>MDYPDPDTIRILITTDNHVGYNENDPITGDDSWKTFHEVMMLAKNNNVDMVVQSGDLFHVNKPSKKSLYQVLKTLRLCCMGDKPCELELLSDPSQVFHYDEFTNVNYEDPNFNISIPVFGISGNHDDASGDSLLCPMDILHATGLINHFGKVIESDKIKVVPLLFQKGSTKLALYGLAAVRDERLFRTFKDGGVTFEVPTMREGEWFNLMCVHQNHTGHTNTAFLPEQFLPDFLDMVIWGHEHECIPNLVHNPIKNFDVLQPGSSVATSLCEAEAQPKYVFILDIKYGEAPKMTPIPLETIRTFKMKSISLQDVPHLRPHDKDATSKYLIEQVEEMIRDANEETKQKLADDGEGDMVAELPKPLIRLRVDYSAPSNTQSPIDYQVENPRRFSNRFVGRVANGNNVVQFYKKRSPVTRSKKSGINGTSISDRDVEKLFSESGGELEVQTLVNDLLNKMQLSLLPEVGLNEAVKKFVDKDEKTALKEFISHEISNEVGILSTNEEFLRTDDAEEMKALIKQVKRANSVRPTPPKENDETNFAFNGNGLDSFRSSNREVRTGSPDITQSHVDNESRITHISQAESSKPTSKPKRVRTATKKKIPAFSDSTVISDAENELGDNNDAQDDVDIDENDIIMVSTDEEDASYGLLNGRKTKTKTRPAASTKTASRRGKGRASRTPKTDILGSLLAKKRKYDYKDDDDKHHHHH[2x];>[2x]MSAIYKLSIQGIRSFDSNDRETIEFGKPLTLIVGMNGSGKTTIIECLKYATTGDLPPNSKGGVFIHDPKITGEKDIRAQVKLAFTSANGLNMIVTRNIQLLMKKTTTTFKTLEGQLVAINNSGDRSTLSTRSLELDAQVPLYLGVPKAILEYVIFCHQEDSLWPLSEPSNLKKKFDEIFQAMKFTKALDNLKSIKKDMSVDIKLLKQSVEHLKLDKDRSKAMKLNIHQLQTKIDQYNEEVSEIESQLNEITEKSDKLFKSNQDFQKILSKVENLKNTKLSISDQVKRLSNSIDILDLSKPDLQNLLANFSKVLMDKNNQLRDLETDISSLKDRQSSLQSLSNSLIRRQGELEAGKETYEKNRNHLSSLKEAFQHKFQGLSNIENSDMAQVNHEMSQFKAFISQDLTDTIDQFAKDIQLKETNLSDLIKSITVDSQNLEYNKKDRSKLIHDSEELAEKLKSFKSLSTQDSLNHELENLKTYKEKLQSWESENIIPKLNQKIEEKNNEMIILENQIEKFQDRIMKTNQQADLYAKLGLIKKSINTKLDELQKITEKLQNDSRIRQVFPLTQEFQRADLEMDFQKLFINMQKNIAINNKKMHELDRRYTNALYNLNTIEKDLQDNQKSKEKVIQLLSENLPEDCTIDEYNDVLEETELSYKTALENLKMHQTTLEFNRKALEIAERDSCCYLCSRKFENESFKSKLLQELKTKTDANFEKTLKDTVQNEKEYLHSLRLLEKHIITLNSINEKIDNSQKCLEKAKEETKTSKSKLDELEVDSTKLKDEKELAESEIRPLIEKFTYLEKELKDLENSSKTISEELSIYNTSEDGIQTVDELRDQQRKMNDSLRELRKTISDLQMEKDEKVRENSRMINLIKEKELTVSEIESSLTQKQNIDDSIRSKRENINDIDSRVKELEARIISLKNKKDEAQSVLDKVKNERDIQVRNKQKTVADINRLIDRFQTIYNEVVDFEAKGFDELQTTIKELELNKAQMLELKEQLDLKSNEVNEEKRKLADSNNEEKNLKQNLELIELKSQLQHIESEISRLDVQNAEAERDKYQEESLRLRTRFEKLSSENAGKLGEMKQLQNQIDSLTHQLRTDYKDIEKNYHKEWVELQTRSFVTDDIDVYSKALDSAIMKYHGLKMQDINRIIDELWKRTYSGTDIDTIKIRSDEVSSTVKGKSYNYRVVMYKQDVELDMRGRCSAGQKVLASIIIRLALSETFGANCGVIALDQPTTNLDEENIESLAKSLHNIINMRRHQKNFQLIVITHDEKFLGHMNAAAFTDHFFKVKRDDRQKSQIEWVDINRVTY

The Mre11 complex is integral to the DNA damage response (DDR). The complex promotes DNA double strand break (DSB) repair and in eukaryotes, it activates the Tel1/ATM kinase to initiate DNA damage signaling. The complex is comprised of two molecules each of Mre11 and Rad50, and one molecule of Nbs1 (Xrs2 in budding yeast). Mre11 and Rad50 (MR) specify enzymatic functions (nuclease and ATPase, respectively), whereas Nbs1/Xrs2 is neither an enzyme, nor does it bind DNA.

To minimize the spatial dynamics of the complex, and to avoid the confounding effects of Xrs2, we next purified the Mre11-Rad50 (MR) complex, in which the E1235 residue of Rad50 was mutated to Q (REQ) to prevent ATP hydrolysis, which likely drives the transition from the closed to the open form of the complex13 15. MREQ was incubated with a 83-mer double stranded DNA (dsDNA) in the presence of ATP, MgCl2 and MnCl2 prior to making the cryo-EM grids. By contrast, traceable coiled coil arm segments of Rad50 (residues 220–239 and 1089–1102) are observed at lower resolution, while the remainder of the coiled coil arm and Zn hook segments (residues 239–1089) of Rad50, the segment (residues 413–441) connecting the capping and HLH domains of Mre11 and the C-terminus of Mre11 (residues 508–692), are flexible and cannot be traced in the complex. In our structure of the S. cerevisiae MR-dsDNA complex, we noted that 18-bp of dsDNA [modeled as an (dA)n-(dT)n duplex] is encapsulated by elements of the pair of Rad50 domains in the MR-dsDNA complex. The dsDNA is positioned above the pair of Rad50 head domains and sandwiched between the pair of Rad50 head-proximal coiled coil arms, anchored in place through a network of hydrogen bonding interactions. We can trace intermolecular hydrogen bonds between Rad50 side chains (-T111, -S169 and -R1201) and main chain (-N58, -F109, -T111 and -S169) with backbone phosphates of bound dsDNA (boxed panel). Notably, the side chain of Rad50-K60 is inserted deep into the minor groove of bound dsDNA and is likely positioned to form hydrogen bonds with bases of dsDNA. Mre11 does not make contacts with the dsDNA, suggesting that this DNA bound structure represents a precursor to the open form of the complex, as predicted previously. The structure of the stable S. cerevisiae MR-dsDNA complex presented here appears to represent a “closed” complex, having a rod-shaped structure that is similar to that recently reported for the C. thermophilum MRN complex in presence of ATPgS, but without DNA11.>[4x]MAKDATQGGVQALSAWTNQSGSTLYIQS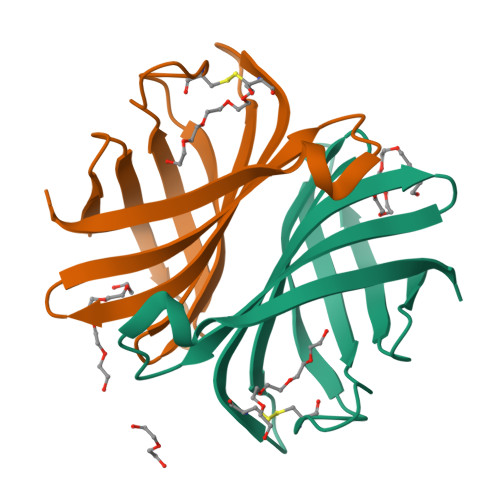VDPSGSLSGYYINRAAGYGCQNTPYPVTGWVYGTAITFTVLWENATESCNSITAWTGFYYQGQITTLWQLVINGSTSTGQIISGEDIFKPS>NLLQFRNMIKCTIPGREPLLAFSNYGCYCGKGGSGTPVDELDRCCQTHDNCYDKAEKLPECKGILSGPYFNTYSYDCTDGKLTCNDQNDKCKLFICNCDRTAAMCFAKAPY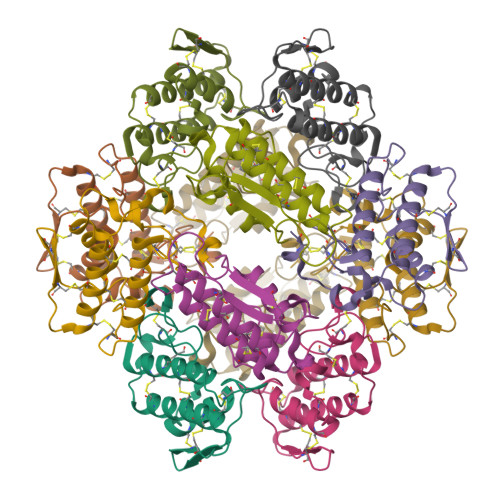NEAYNHFNRQLCK[6x]>GEIQWMRPSKEVGYPIINAPSKTKLEPSAFHYVFEGVKEPAVLTKNDPRLKTDFEEAIFSKYVGNKITEVDEYMKEAVDHYAGQLMSLDIN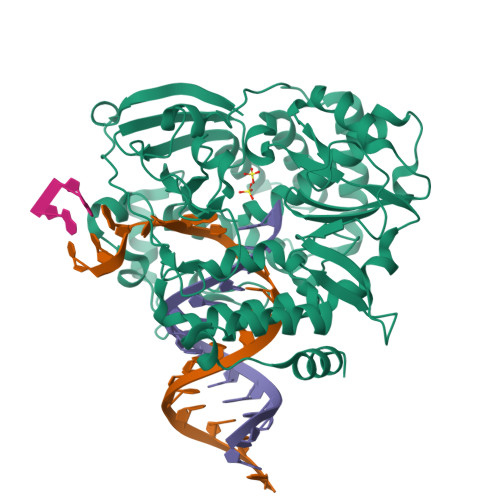TEQMCLEDAMYGTDGLEALDLSTSAGYPYVAMGKKKRDILNKQTRDTKEMQKLLDTYGINLPLVTYVKDELRSKTKVEQGKSRLIEASSLNDSVAMRMAFGNLYAAFHKNPGVITGSAVGCDPDLFWSKIPVLMEEKLFAFDYTGYDASLSPAWFEALKMVLEKIGFGDRVDYIDYLNHSHHLYKNKTYCVKGGMPSGMSGTSIFNSMINNLIIRTLLLKTYKGIDLDHLKMIAYGDDVIASYPHEVDASLLAQSGKDYGLTMTPADKSATFETVTWENVTFLKRFFRADEKYPFLIHPVMPMKEIHESIRWTKDPRNTQDHVRSLCLLAWHNGEEEYNKFLAKIRSVPIGRALDLPEYSTLYRRWLDSFGSSSHHHHHH[2x]> DYLFKVVLIGDSGVGKSNLLSRFTRNEF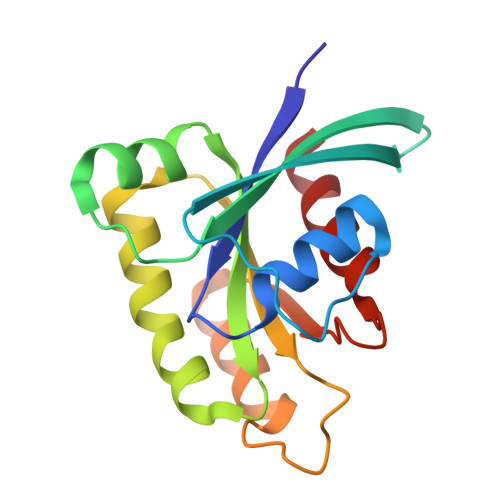NLESKSTIGVEFATRSIQVDGKTIKAQIWDTAGQERYRAITSAYYRGAVGALLVYDIAKHLTYENVERWLKELRDHADSNIVIMLVGNKSDLRHLRAVPTDEARAFAEKNGLSFIETSALDSTNVEAAFQTILTEIY>GSGSELARKLLEASTKLQRLNIRLAEALLEAIARLQELNLELVYLAVELTDPKRIRDEIKEVKDKSKEIIRRAEKEIDDAAKESEKILEEAREAISGSGSELAKLLLKAIAETQDLNLRAAKAFLEAAAKLQELNIRAVELLVKLTDPATIREALEHAKRRSKEIIDEAERAIRAAKRESERIIEEARRLIEKGSGSGSELARELLRAHAQLQRLNLELLRELLRALAQLQELNLDLLRLASELTDPDEARKAIARVKRESNAYYADAERLIREAAAASEKI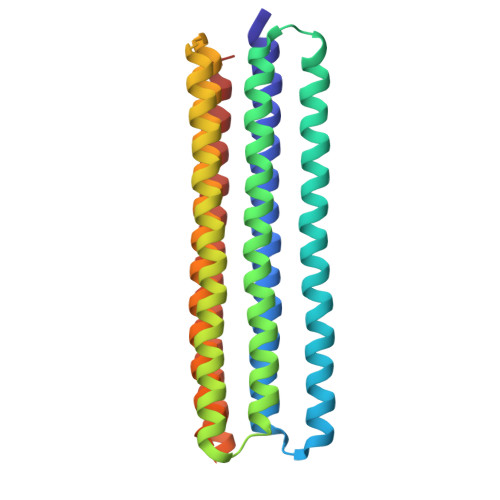SREAERLIR[2x]CEFOXITIN | C16 H17 N3 O7 S2 | 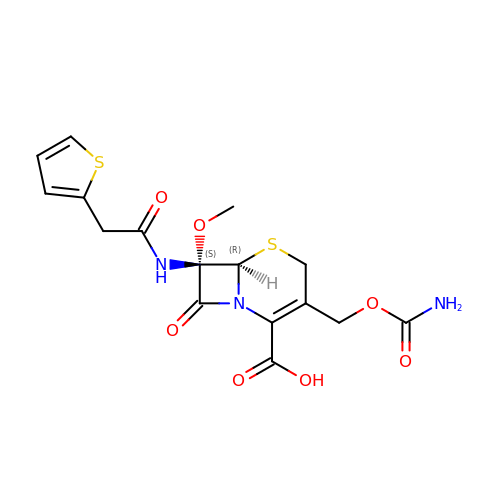WZOZEZRFJCJXNZ-ZBFHGGJFSA-N>GDHIKVIYFNGRGRAESIRMTLVAAGVNYEDERISFQDWPKIKPTIPGGRLPAVKITDNHGHVKWMLESLAIARYMAKKHHMMGETDEEYYNVEKLIGQVEDLEHEYHKTLMKPEEEKQKITKEI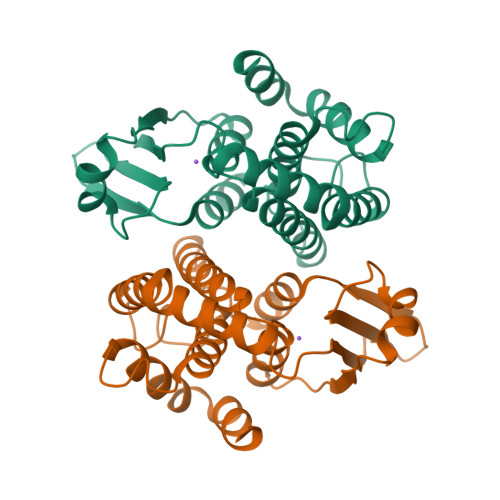LNGKVPVLLDIICESLKASTGKLAVGDKVTLADLVLIAVIDHVTDLDKEFLTGKYPEIHKHRENLLASSPRLAKYLSDRA[2x]>[2x]MEQEKVQELVSQMTLDEKIAQCLQLSPFLFKGTNKNAELTGPLLQEMKLTDAHTENAGSVLGSSSALDMIGIQEAYLKTNRLGIPLVFMADVIHGYKTVFPIPLALGCSFDRETVRVMAEVSALEATADGHHVTFSPMLDLVRDPRWGRVMESTGEDPFLNSELGKAMVDGYQGDASKLNENLEQMAACVKHFAAYGAAEAGLEYNTVNMSTRELYQNYLPAYNAAIQAGAKLVMTAFNVVDGIPATMNKWLNRDVLRGEMEFDGVLISAWGAVAEVINHGTARNPKEAAQFSMEAGVDLEMMTTCYIHELKGLIEEGKLSENLLDEAVLRMLNLKNDLGLFEDPYRGLKNNDRTKDILTDESRGKARAAGVESAVLLENKSRLLPLAKEAKIALVGPLATSPDILGGWNVYGEEKDGINVETGLREVFETVEVVSTEYTELSEEDKVAVKAAVQNMDVVVLALGEKNEWGGEAGSLATIRLPEAQYQLAKFVQTLGKPVVITLFNGRPLEVKELAESSDALLELWFPGTEAGRVTADLLSGASNPSGKLSMSFPQTTGQIPVYYNHLRTGRPQTPENKGERYVSHYLDIPNEPFYPFGYGKSYSEFELKTSSLPKELNLGESLHVEVTIKNISDIAGKEVIQVYLQDVTASISRPVKELKAFEKVALQAGEEKTVTFELTSEAFSFYNHQLEKVQEPGLHRVFVGTSSEDVDVFEVEVGGYVLEHHHHHH

In the gene cluster containing the lin1839 gene, the lin1840 gene encodes a putative glycoside hydrolase family (GH) 3 β-glucosidase (BGL) (GenBank accession number: CAC97071.1). The structure showed that Lin1840r forms a dimer of identical subunits each composed of three domains. The active center of Lin1840r is located at the interface of domains 1 and 2 as in the cases of known GH3 BGLs.

In order to understand the recognition mechanism of Sop2 and Lam2, the complex structures with these disaccharides were determined using the nucleophile D270A mutant of Lin1840r. The electron density of Sop2 was clearly observed in the D270A structure on soaking in 100 mM Sop2 and fitted only with the β-anomer. The Glc moieties of both Sop2 and Lam2 at subsite −1 are located at almost the same positions as the ligands in WT-inhibitors complexes despite the replacement of the catalytic nucleophile with alanine. The reducing end Glc moieties of Sop2 and Lam2 are consistently stacked on Trp271 and Tyr583, and form four hydrogen bonds with Arg572, suggesting that these three residues constitute subsite +1. The fact that Tyr583 and Arg572 are derived from a loop in the adjacent subunit indicates the participation of both subunits in formation of the catalytic pocket. Sop2 complex is also considered as Michaelis complex in spite of its conformation, since Sop2 is not superimposed with glucophenylimidazole (PheGlcIm) known as a transition-like analog in HvExoI but with ligands known as Michaelis complex, such as 2',4'-dinitrophenyl-2-deoxy-2-fluro-β-d-cellobioside (Cel2F-DNP) in GH5 Bacillus agaradhaerens endo-β-1,4-glucanase (BaCel5A), a retaining enzyme. In the Sop2 and Lam2 complexes, the angles defined by the oxygen atom of the glycosidic bond, the anomeric carbon atoms in the ligands, and the carboxyl group in the catalytic nucleophile are 165° and 164°, respectively, as in the case of GlcNAc-MurNAc in a nucleophile mutant of GH3 B. subtillus N-acetyl-β-d-glucosaminidase and Cel2F-DNP in BaCel5A. The distances between the catalytic nucleophile and the anomeric carbon at subsite −1 are 3.2 Å and 3.0 Å, respectively, and the distances between the catalytic acid-base and oxygen atoms of the glycosidic bond are 3.4 Å and 3.2 Å, respectively. The anomeric hydroxy group of reducing end glucosides in Sop2 is exposed to the solvent, in the vicinity of Asp91.>[2x]MNGRGFLIYNGGEKMKQKMIIYDTPAGPYPA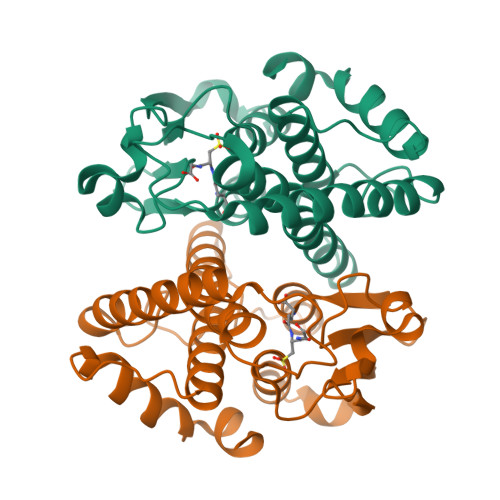RVRIALAEKNMLSSVQFVRINLWKGEHKKPEFLAKNYSGTVPVLELDDGTLIAECTAITEYIDALDGTPTLTGKTPLEKGVIHMMNKRAELELLDPVSVYFHHATPGLGPEVELYQNKEWGLRQRDKALHGMHYFDTVLRERPYVAGDSFSMADITVIAGLIFAAIVKLQVPEECEALRAWYKRMQQRPSVKKLLEIRSKSS>GPHMLDLFADAEPWQEPLAAGAVILRRFAFNAAEQLIRDINDVASQSPFRQMVTPGGYTMSVAMTNCGHLGWTTHRQGYLYSPIDPQTNKPWPAMPQSFHNLCQRAATAAGYPDFQPDACLINRYAPGAKLSLHQDKDEPDLRAPI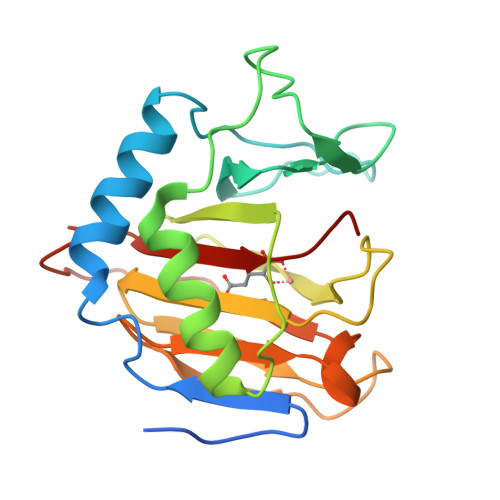VSVSLGLPAIFQFGGLKRNDPLKRLLLEHGDVVVWGGESRLFYHGIQPLKAGFHPLTIDCRYNLTFRQAGKKE[2x]> SGRPMDNEEWFPLKQTHYPPPTIPSMKTGHPTGPI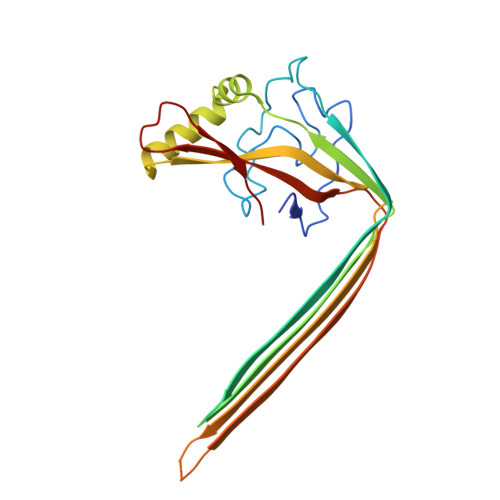SIGHIIPDLRHLDNVINCKGFEPFPPNMDVFTAHYEQCHFGDHLNSEFVVQAKAAAPIENIVPGVDVTGSAGLHHTNITSDRWEYDSVVEYAVYPTRQYIDRLLESKEVRQYIQKSKKLLGGWCVYMVTGIMVARGGGRNVTSEEKGAGVSGNVGFQVPGIGEFAPEVGWDTKTKTKVNAHHTTDFVCAIRLVKIAKSGLRSSWTMKKVTREF> SAVRPTKRIEFTEADGDTEGKSVFQLEKETDKETFKIRDDNPWVTVETNGAVRVKKKWDYEELGPEKTIDFWVIITNMGHNAGIKYTDNQRVIILVKDVNDEPPYFINRPLPMQAVVQLNAPPNT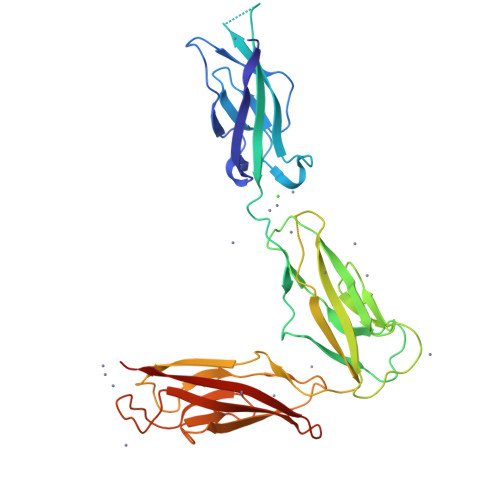PVFTLQARDPDTDHNIHYFIVRDRTGGRFEVDERSGVVRTRGTDLFQLDMEYVLYVKAEDQNGKVDDRRFQSTPEERLSIVGGKRAPQFYMPSYEAEIPENQKKDSDIISIKAKSFADREIRYTLKAQGQGAGTFNIGPTSGIVKLAKELDFEDLRQPHVYSLIVTATEDSGGFSTSVDLTIRVTDVNDNA> MSKEIPTPYMWSYQPQMGLAAGAAQDYSTRINYMSAGPHMISRVNGIRAHRNRILLEQAAITTTPRNNLNPRSWPAALVYQESPAPTTVVLPRDAQAEVQMTNSGAQLAGGFRHRVRSPGQGITHLTIRGRGIQLNDESVSSSLGLRPDGTFQIGGAGRPSFTPRQAILTLQTSSSEPRSGGIGTLQFIEEFVPSVYFNP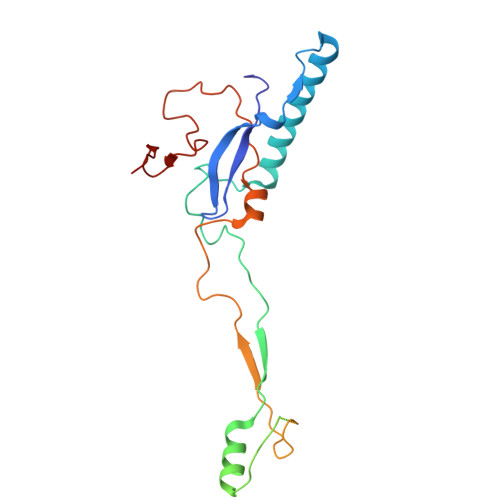FSGPPGHYPDQFIPNFDAVKDSADGYD> GPGSMAASRRLMKELEEIRKCGMKNFRNIQVDEANLLTWQGLIVPDNPPYDKGAFRIEINFPAEYPFKPPKITFKTKIYHPNIDEK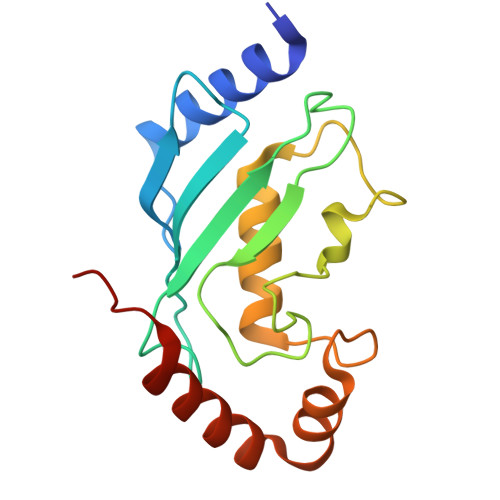GQVCLPVISAENWKPATKTDQVIQSLIALVNDPQPEHPLRADLAEEYSKDRKKFCKNAEEFTKKYGEKRPVD> MQRQAGLPLKANPMHTIASILLSVLGIYSPADVAGLPTHLYKNFTVQELALKLKGKNQEFCLTAFM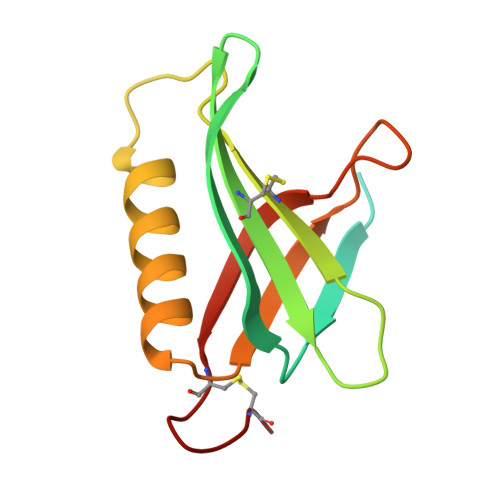SGRSLVRACLSDAGHEHDTWFDTMLGFAISAYALKSRIALTVEDSPYPGTPGDLLELQICPLNGYCE Autophagosome formation is a fundamental process in macroautophagy/autophagy, a conserved self-eating mechanism in all eukaryotes, which requires the conjugating ATG (autophagy related) protein complex, ATG12–ATG5-ATG16L1 and lipidated MAP1LC3/LC3 (microtubule associated protein 1 light chain 3). Here, we demonstrated that RAB33B plays a key role in recruiting the ATG16L1 complex to phagophores during starvation-induced autophagy. Crystal structures of RAB33B bound to the coiled-coil domain (CCD) of ATG16L1 revealed the recognition mechanism between RAB33B and ATG16L1. ATG16L1 is a novel RAB-binding protein (RBP) that can induce RAB proteins to adopt active conformation without nucleotide exchange.

We prepared the ATG16L1(141–265) complexes with GDP-bound RAB33B(30–218) or GTP-bound RAB33BQ92L(30–218). Their crystal structures were determined at 2.4 Å. To our surprise, both GDP- and GTP-bound RAB33B adopted the same conformation in the complexes. Structural comparison of GTP- and GDP-bound RAB33B molecules in complexes with ATG16L1 revealed that their conformations are identical with an alpha-carbon root-mean square deviation (Cα-RMSD) of 0.16 Å. The conformations of GTP- and GDP-bound RAB33B complexes remained identical at the switch I and switch II regions, where the major conformational changes are typically observed in different nucleotide binding states. ATG16L1 binding induced a remarkable conformational change of the switch I region. This results in a ca. 8.4 Å translocation of the Cα atom of I66, followed by a hydrophobic packing of I66 against F95 of RAB33B and W194 of ATG16L1. The switch II region is largely disordered in GDP-bound RAB1A, while the switch II region of RAB33B adopted the active conformation and formed extensive interactions with ATG16L1. Therefore, ATG16L1 induced conformational changes of GDP-bound RAB33B to hold it in the active conformation. Importantly, E186 and R193 in the other molecule of the dimeric ATG16L1 contributed to the stabilization of the active conformation of GDP-RAB33B via hydrogen bonding with R94 of the switch II region and the main chain of the switch I region, respectively.

>[2x]GPMRSRIFKIIVIGDSNVGKTCLTYRFCAGRFPDRTEATIGVDFRERAVEIDGERIKIQLWDTAGQERFRKSMVQHYYRNVHAVVFVYDMTNMASFHSLPSWIEECKQHLLANDIPRILVGNKCDLRSAIQVPTDLAQKFADTHSMPLFETSAKNPNDNDHVEAIFMTLAHKLKSHKPLMLSQPPDNGIILK;>MLETNCLDLRTKLQDLEVANQTLKDEYDALQITFTALEEKLRKTTEENQELVTRWMAEKAQEANRLNAENEKDSRRRQARLQKELAEAAKEPLPVEQDDDIEVIVDETSDHTEETSPVRAVSRAAT[2x]> MGLFDRIKRVVSSNLNDLVNKAEDPEKMLEQAILEMQE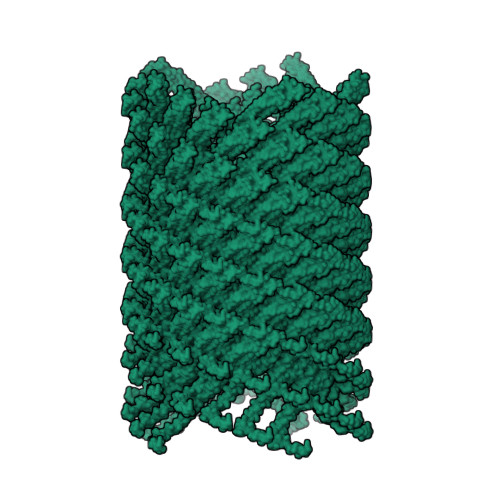DLVQLRQGVAQAIAAQKRSEKQYNDAQNEINKWQRNAQLALQKGDENLARQALERKKTYTDTSAALKASLDTQSTQVETLKRNLIQLESKISEAKTKKEMLKARITTAKAQEQLQGMVRGMNTSSAMSAFERMEEKVLMQESRAQALGELAGADLETQFAQLEGGSDVDDELAALK>[4x]SPLHFAASYGRINTCQRLLQDISDTRLLNEGDLHGMTPLHLAAKNGHDKVVQLLLKKGALFLSDHNGWTALHHASMGGYTQTMKVILDTNLKCTDRLDEDGNTALHFAAREGHAKAVALLLSHNADIVLNKQQASFLHLALHNKRKEVVLTIIRSKRWDECLKIFSHNSPGNKCPITEMIEYLPECMKVLLDFCMLHSTEDKSCRDYYIEYNFKYLQCPLEFTKKTPTQDVIYEPLTALNAMVQNNRIELLNHPVCKEYLLMKWLAYGFRAHMMNLGSYCLGLIPMTILVVNIKPGMAFNSTGIINETSDHSEILDTTNSYLIKTCMILVFLSSIFGYCKEAGQIFQQKRNYFMDISNVLEWIIYTTGIIFVLPLFVEIPAHLQ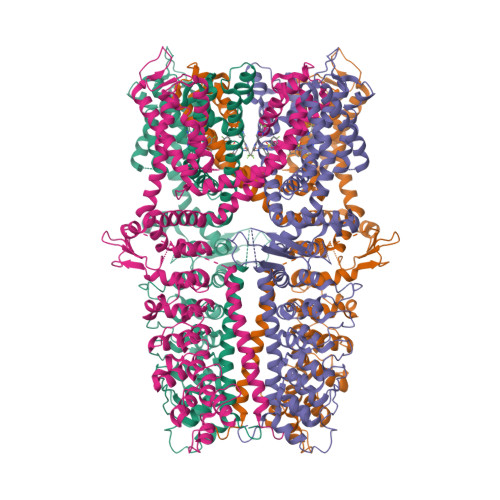WQCGAIAVYFYWMNFLLYLQRFENCGIFIVMLEVILKTLLRSTVVFIFLLLAFGLSFYILLNLQDPFSSPLLSIIQTFSMMLGDINYRESFLEPYLRNELAHPVLSFAQLVSFTIFVPIVLMNLLIGLAVGDIADVQKHASLKRIAMQVELHTSLEKKLPLWFLRKVDQKSTIVYPNKPRSGGMLFHIFCFLFCTGEIRQEIPNADKSLEMEILKQKYRLKDLTFLLEKQHELIKLIIQKMEIISET> MTHSSQRRILLLAAAAAPLALSVGACAARD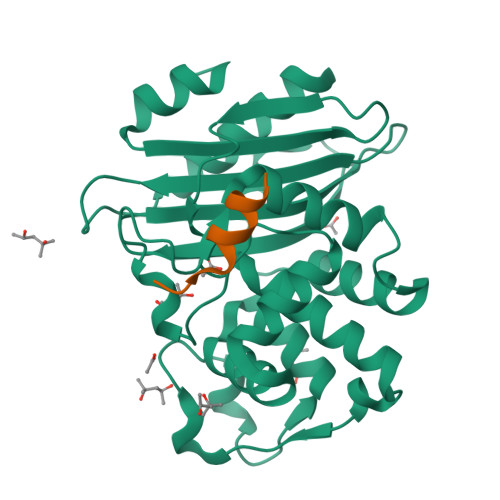AAVSDAASPVGAAPASFAALERAAGGRLGVCAIDTATGRRTLHRADERFPFCSTFKAMLGAAVLAQSVAHPGLLQQRVTYGRSDLVSYSPVTERHVDTGMTVAELCAATIQYSDSTAANELMKLIGGPAAVTAYARSIGDDTFRLDRWETELNTALPGDLRDTTTPAAMAASLRVLVLGDALPAAQRAQLIEWLRGNKVGDKRIRAGVPTGWRVGDKTGTGDYGTTNDAGVLWPPSRAPIVLAVYYTQTRADAKAKDDVIATATRIAIATLG;> AARDAAVSDAAA>[2x]EVDPRLYFENRSKFIQDQKDKGINPYPHKFERTISIPEFIEKYKDLGNGEHLEDTILNITGRIMRVSASGQKLRFFDLVGDGEKIQVLANYSFHNHEKGNFAECYDKIRRGDIVGIVGFPGKSKKGELSIFPKETILLSACLHMLPMKYGLKDTEIRYRQRYLDLLINESSRHTFVTRTKIINFLRNFLNERGFFEVETPMMNLIAGGANARPFITHHNDLDLDLYLRIATELPLKMLIVGGIDKVYEIGKVFRNEGIDNTHNPEFTSCEFYWAYADYNDLIKWSEDFFSQLVYHLFGTYKISYNKDGPENQPIEIDFTPPYPKVSIVEEIEKVTNTILEQPFDSNETIEKMINIIKEHKIELPNPPTAAKLLDQLASHFIENKYNDKPFFIVEHPQIMSPLAKYHRTKPGLTERLEMFICGKEVLNAYTELNDPFKQKECFKLQQKDREKGDTEAAQLDSAFCTSLEYGLPPTGGLGLGIDRITMFLTNKNSIKDVILFPTMRPAN

Aminoacyl-tRNA synthetases catalyze aminoacylation of tRNAs with their cognate amino acids in two stages. First, the amino acid is activated by ATP to yield the AMP-activated amino acid, with loss of pyrophosphate, followed by transfer of the amino acid onto the tRNA. Malaria parasite genomes encode two different lysyl-tRNA synthetases (KRSs) that play a role in translation in either the cytoplasm (PfKRS1) or in the apicoplast (PfKRS2), while Cryptosporidium parasites and humans encode one copy. We present a selective inhibitor of both Plasmodium and Cryptosporidium lysyl-tRNA synthetase capable of clearing parasites from mouse models of malaria and cryptosporidiosis infection.

Addition of fluorines on the 4-position of the cyclohexyl ring in 5 was tolerated and led to excellent metabolic stability, both in mouse and human liver microsomes. The complex of 5 bound to PfKRS1 showed that the addition of the difluoro moiety on the cyclohexyl ring had minimal effect upon the position of the ligand within the binding site with respect to 4, and there was no evidence of protein rearrangement. In this complex, all polar interactions were retained, although the H-bond between the bridge-head OH and the side chain of Glu-500 had shortened to 3.0 Å. Compound 5 was active against both PfKRS1 (IC50 = 0.015 μM) and whole-cell bloodstream P. falciparum 3D7 (EC50 = 0.27 μM) and was selective compared with both the HsKRS (IC50 = 1.8 μM) and HepG2 cells (EC50 = 49 μM). Under our experimental conditions, results showed a linear competitive inhibition vs. ATP with a Ki of 32 nM and a linear uncompetitive inhibition vs. l-lysine with a Ki of 212 nM. These results indicate that compound 5 competes with ATP for the same binding site and only binds in the presence of l-lysine, also suggesting a sequential ordered kinetic mechanism where l-lysine is the first substrate to bind. Molecular dynamics (MD) simulations were successful in reproducing the binding pose and interactions of compound 5 observed in the co-crystal structure of PfKRS1. In addition to those interactions, the inhibitor was found to be stabilized by hydrophobic contacts established between the cyclohexyl moiety and the bound substrate l-lysine. Simulations performed in the absence of l-lysine showed a notable destabilization of compound 5, suggesting a key role of l-lysine in the binding of PfKRS1 inhibitors. In apo-PfKRS1, due to the smaller size of V328 and S344 side chains, the ligand binding pocket remained accessible to compound 5.>MKIRDLLKARRGPLFSFEFFPPKDPEGEEALFRTLEELKAFRPAFVSITYGAMGSTRERSVAWAQRIQSLGLNPLAHLTVAGQSRKEVAEVLHRFVESGVENLLALRGDPPRGERVFRPHPEGFRYAAELVALIRERYGDRVSVGGAAYPEGHPESESLEADLRHFKAKVEAGLDFAITQLFFNNAH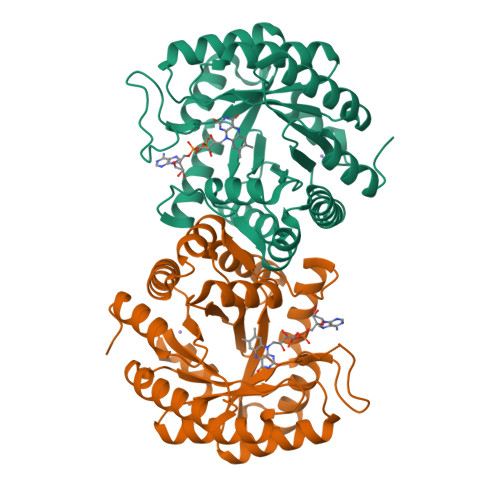YFGFLERARRAGIGIPILPGIMPVTSYRQLRRFTEVCGASIPGPLLAKLERHQDDPKAVLEIGVEHAVRQVAELLEAGVEGVHFYTLNKSPATRMVLERLGLRPASGQP[2x]> GGSYSKSPSNKDAALLEAARANNMQEVSRLLSEGADVNAKHRLGWTALMVAAINRNNSVVQVLLAAGADPNLGDDFSSVYKTAKEQGIHSLEDGGQDGASRHITNQWTSALEFRRWLGLPAGVLITREDDFNNRLNNRASFKGCTALHYAVLADDYRTVKELLDGGANPLQRNEMGHTPLDYAREGEVMKLLRTSEAKYQEKQRKREAEERRRFPLEQRLKEHIIGQESAIATVGAAIRRKENGWYDEEHPLVFLFLGSSGIGKTELAKQTAKYMHKDAKKGFIRLDMSEFQERHEVAKFIGSPPGYVGHEEGGQLTKKLKQCPNAVVLFDEVDKAHPDVLTIMLQLFDEGRLTDGKGKTIDCKDAIFIMTSNVASDEIAQHALQLRQEALEMSRNRIAENLGDVQISDKITISKNFKENVIRPILKAHFRRDEFLGRINEIVYFLPFCHSELIQLVNKELNFWAKRAKQRHNITLLWDREVADVLVDGYNVHYGARSIKHEVERRVVNQLAAAYEQDLLPGGC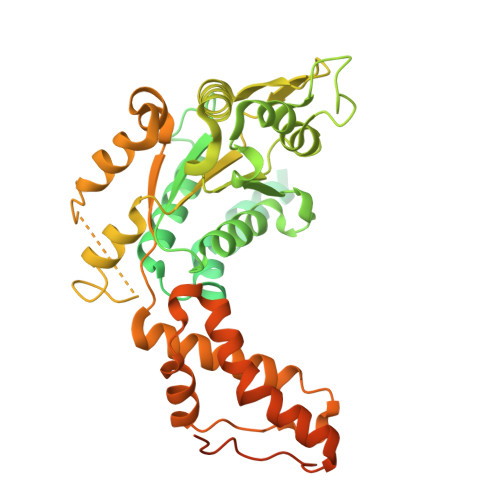TLRITVEDSDKQLLKSPELPSPQAEKRLPKLRLEIIDKDSKTRRLDIRAPLHPEKVCNTI3-(4-HYDROXY-PHENYL)PYRUVIC ACID | C9 H8 O4 | 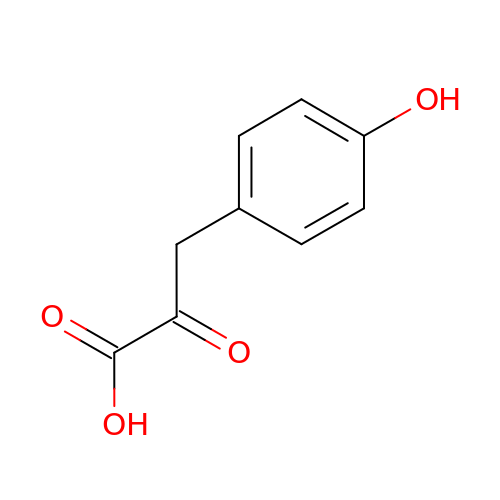KKADPXVIOXHVKN-UHFFFAOYSA-N>MNDNVAWFKQAKYGMMIHWGLYSLLAGEYRGESSSAYAEWIQSKFQIPNAEYGNLATAFNPLYFDAKKIVALAKQCGMQYLVVTTKHHDGFAMYHSKVDAYNVYDATPFHRDIIGELAEACQKAGLKFGLYYSQDLDWHDPNGGGYKSNDVETAGTTWDNSWDFPDEDQKNFDLCFDNKILPQIKEIMSNYGDIATAWFAVPMTLSEAQSQTIYDTVRELQPNCLINSRLGNGKYDFVSLGDNEIPKNKEDMNKTDVDYNEITGFKPSPLGLYETAGTINDSWGFSYHDQNWKTPRTLYRYKQHLNDFGINYLLNVGLDPLGRVPMMAEENLLAAKALEDEANRL[8x]

Lactobacillus casei produces a GH29A α-fucosidase, AlfC, that is ~104-fold more active on α(1-6)-fucosyl linkages compared to other linkages. This enzyme is particularly relevant because α(1-6) linkages form the basis of human core fucosylation, which significantly impacts the function of glycoproteins such as antibodies. AlfC is a single-domain enzyme that adopts a (β/α)8 fold typical of GH29 enzymes, with an active site at the center of the barrel. Our results suggest that AlfC employs a conserved hydrolytic mechanism with a specific subsite that accommodates GlcNAc in α(1,6)-linkages, while AlfC tranfucosidase mutants work by shifting equilibrium between open and closed conformations of an active-site loop.

We soaked this substrate into apo AlfCD200A crystals and observed clear electron density for it. However, despite the bound substrate, we observed no conformational changes in any of the acid/base candidates, and the Cα of D200A and D242 were still ~16.5 Å apart. 4NP-fuc bound in an orientation nearly identical to that seen in BT2970, where the Cα of the nucleophile and acid/base are separated by ~12.5 Å, in a conformation compatible with catalysis. In BiAfcB, it has been observed that the Cα of the acid/base can move from ~17.6 Å away from the nucleophile Cα, to only ~12.1 Å away. The same conformational change in AlfC would place the Cα of D242 only ~11 Å from the nucleophile Cα, in a position compatible with catalysis. Therefore, structural homology suggests the existence of open and closed states of AlfC.>MHHHHHHTDPALRAAELLLGVNIDHIATLRNARGTAYPDPVQAAFIAEQAGADGITVHLREDRRHITDRDVRILRQTLDTR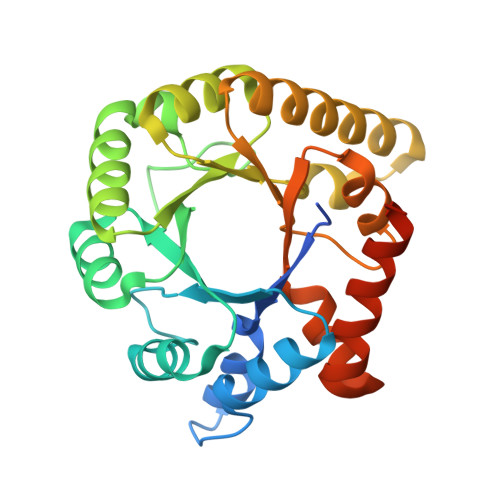MNLEMAVTEEMLAIAVETKPHFCCLVPEKRQEVTTEGGLDVAGQRDKMRDACKRLADAGIQVSLFIDADEEQIKAAAKVGAPFIEIHTGCYADAKTDAEQAQELARIAKAATFAASLGLKVNAGHGLTYRNVKAIAAIPEMHELNIGHAIIGRAVLTGLKVAVAEMKRLMLEARGGLEPLRVVSLIS[4x]> LRPGDCEVCISYLG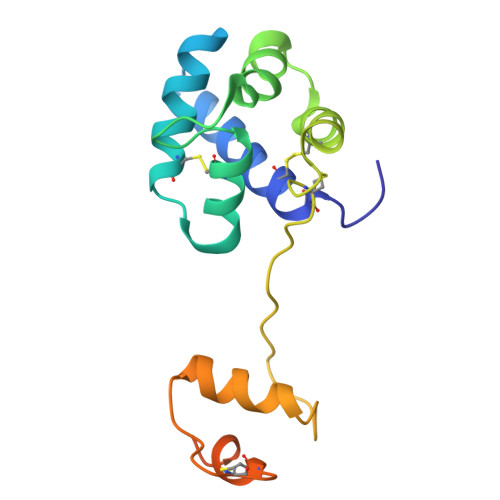RFYQDLKDRDVTFSPATIENELIKFCREARGKENRLCYYIGATDDAATKIINEVSKPLAHHIPVEKICEKLKKKDSQICELKYDKQIDLSTVDLKKLRVKELKKILDDWGETCKGCAEKSDYIRKINELMPKYAPKAASARTDL4-[1-[3-[4-[(4-fluoranyl-2-methyl-1H-indol-5-yl)oxy]-6-methoxy-quinazolin-7-yl]oxypropyl]piperidin-4-yl]benzamide | C33 H34 F N5 O4 | 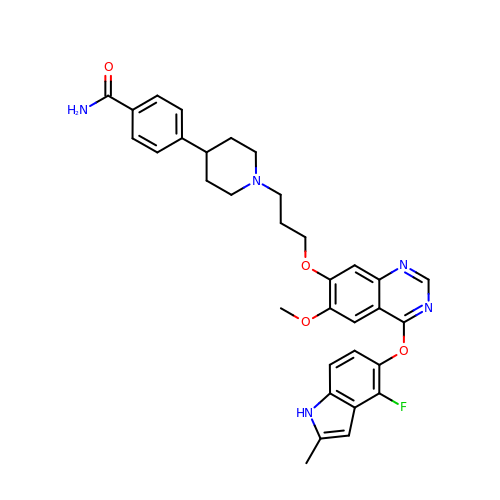ZUKPQXRSZJTISJ-UHFFFAOYSA-N>[6x]MALISQSIKNLKGGISQQPDILRYPDQGSRQVNGWSSETEGLQKRPPLVFLNTLGDNGALGQAPYIHLINRDEHEQYYAVFTGSGIRVFDLSGNEKQVRYPNGSNYIKTANPRNDLRMVTVADYTFIVNRNVVAQKNTKSVNLPNYNPNQDGLINVRGGQYGRELIVHINGKDVAKYKIPDGSQPEHVNNTDAQWLAEELAKQMRTNLSDWTVNVGQGFIHVTAPSGQQIDSFTTKDGYADQLINPVTHYAQSFSKLPPNAPNGYMVKIVGDASKSADQYYVRYDAERKVWTETLGWNTEDQVLWETMPHALVRAADGNFDFKWLEWSPKSCGDVDTNPWPSFVGSSINDVFFFRNRLGFLSGENIILSRTAKYFNFYPASIANLSDDDPIDVAVSTNRIAILKYAVPFSEELLIWSDEAQFVLTASGTLTSKSVELNLTTQFDVQDRARPFGIGRNVYFASPRSSFTSIHRYYAVQDVSSVKNAEDITSHVPNYIPNGVFSICGSGTENFCSVLSHGDPSKIFMYKFLYLNEELRQQSWSHWDFGENVQVLACQSISSDMYVILRNEFNTFLARISFTKNAIDLQGEPYRAFMDMKIRYTIPSGTYNDDTFTTSIHIPTIYGANFGRGKITVLEPDGKITVFEQPTAGWNSDPWLRLSGNLEGRMVYIGFNINFVYEFSKFLIKQTADDGSTSTEDIGRLQLRRAWVNYENSGTFDIYVENQSSNWKYTMAGARLGSNTLRAGRLNLGTGQYRFPVVGNAKFNTVYILSDETTPLNIIGCGWEGNYLRRSSGI

Escherichia coli bacteriophage T7, a member of Podoviridae, has been used as a model for understanding the DNA packaging mechanism common to tailed phages and related dsDNA viruses. The phages package genomic dsDNA into a round procapsid using the portal in complex with an ATP-dependent terminase complex as the motor. At the beginning of phage infection, the tail is responsible for receptor recognition, and the portal and tail act as a tunnel for DNA delivery into the host cytoplasm. Here, we determined structures of the DNA packaging intermediate and mature capsids of T7 using cryo-electron microscopy (cryo-EM) and symmetry-mismatch reconstruction.

Subsequently, a 7 Å resolution asymmetric reconstruction of the mature phage with a portal-tail complex at one of the 12 icosahedral vertices was obtained using the symmetry-mismatch reconstruction method. The portal-tail complex structure is similar to the previously reported recombinant T7 portal-tail complex structure. The portal-tail complex was reconstructed at the same resolution of 3.8 Å, although the core structure was still smeared. Another two independent local reconstructions focused on the portal and tail, respectively, yield the structures of the portal and tail at the same resolution of 3.8 Å, suggesting that the portal interacts firmly with the tail. Twelve copies of adaptor protein gp11 assemble around the bottom of the portal forming a ring-like structure and serving as the base for the assembly of a hexameric tube consisting of six copies of nozzle protein gp12. The dsDNA is embraced by the 12 tunnel loops in the portal, which have a weaker density probably due to its asymmetric interaction with the dsDNA groove. This dsDNA density terminates abruptly at the interface between the dodecameric ring of gp11 and hexameric nozzle of gp12. Consequently, the terminase complex cleaves the mature DNA genome from the concatemer and disassociates from the portal clip, followed by the association of the tail adaptor and nozzle to complete the phage assembly.>DKGKLSLQDVAELIRARACQRVVVMVGAGISTPSGIPDFRSPGSGLYSNLQQYDLPYPEAIFELPFFFHNPKPFFTLAKELYPGNYKPNVTHYFLRLLHDKGLLLRLYT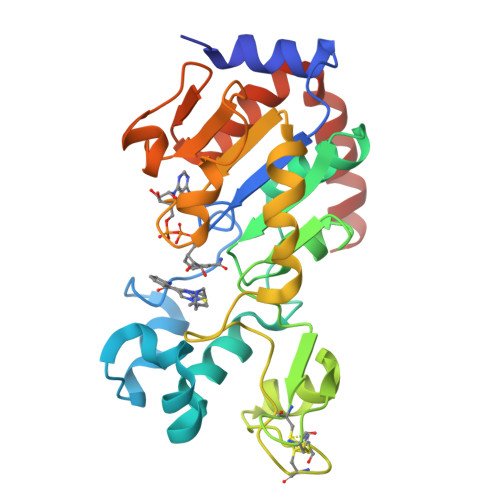QNIDGLERVSGIPASKLVEAHGTFASATCTVCQRPFPGEDIRADVMADRVPRCPVCTGVVKPDIVFFGEPLPQRFLLHVVDFPMADLLLILGTSLEVEPFASLTEAVRSSVPRLLINRDLVGPLAWHPRSRDVAQLGDVVHGVESLVELLGWTEEMRDLVQRETGKLDGPDK[12x]> MESSSSLKGSALGKLVVTSGLLHSSWSKILEIHNPPYSNHDPGLQVSKKKKDSGLEFQIHREEKFTLVVFSAPPICRSSSSDSTLLHVKDKENPFPFLCSENNPSFSLHTPAFNLFTSASTSLTYLKSELLQTLKSEKPVIITGAALGGSVASLYTLWLLETIEPTLKRPLCITFGSPLIGDASLQQILENSVRNSCFLHVVSAQTRIKMDFFKPFGTFLICFDSGCVCIEDHVAVTELLNGVHDSGLVDYSQVLNRLDQSMLSLA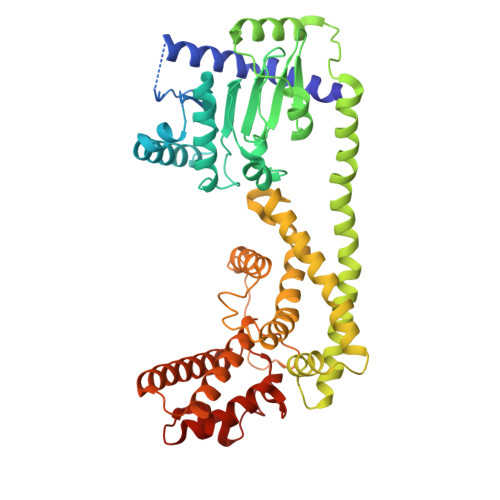DSRLIPEDVIKGIEKRAEMKNLRFDMMFKKLNDMKISMAYIEWYKKKCKEVKIGYYDRFKTQLAFPSKEFDINIKNHHKSELNRFWKSVVEEVERRPQSDASILKRRFLFSGNNYRRMIEPLDIAEYYLEGRKEYRTTGRSHHYVMLEKWFGMESILIEKERCKKRDLSDLLTFDSCFWAEVEDSLIVINQLNTTVGMRDDVREVLTRKLVEFEGYVWEIITKREVSPEIFLEESSFMKWWKEYKKIKGFNSSYLTEFMNTRKYESYGKSQ>[4x]GPYASLTEIEHLVQSVCKSYRETCQLRLEDLLRQRSNIFSREEVTGYQRKSMWEMWERCAHHLTEAIQYVVEFAKRLSGFMELCQNDQIVLLKAGAMEVVLVRMCRAYNADNRTVFFEGKYG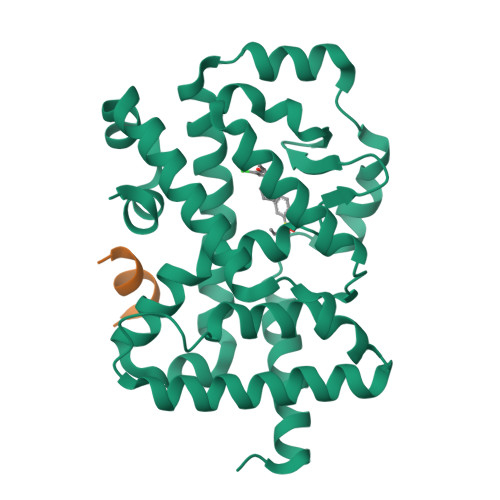GMELFRALGCSELISSIFDFSHSLSALHFSEDEIALYTALVLINAHRPGLQEKRKVEQLQYNLELAFHHHLSKTHRQSILAKLPPKGKLRSLCSQHVERLQIFQHLHPIVVQAAFPPLYKELFSTETESPVGLSK;>NSHQKVTLLQLLLGHKNEEN[4x]> MSVDRYSGMEGTEHIRFQRLVQVCNKALEESIRKLQSWEKIHECFPNYGQTREGIENLTVCQQQVIKLWSNLSRVEFDAIFHERSIEEKLNQLDDLINKARSIDTSSSSKKLRKIDDLRP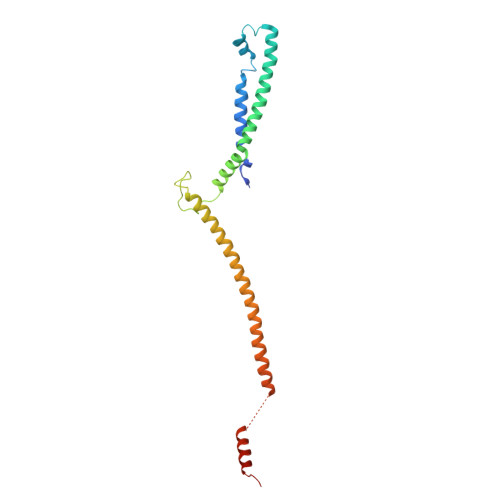LELIEGNLQGAKESTLERINNKLQIIKESNEALETNLKDLNDNIFQELDQLQQVYDDMLNEKSMLPDETIKQAVSDMIIESRQTS> MHRRGVGAGAIAKKKLAEAKYKERGTVLAEDQLAQMSKQLDMFKTNLEEFASKHKQEIRKNPEFRVQFQDMCATIGVDPLASGKGFWSEMLGVGDFYYELGVQIIEVCLALKHRNGGLITLEELHQQVLKGRGKFAQDVSQDDLIRAIKKLKALGTGFGIIPVGGTYLIQSVPAELNMDHTVVLQLAEKNGYVTVSEIKASLKWETERARQVLEHLLKEGLAWLDLQAPGEAHYWLPALFTDLYSQEI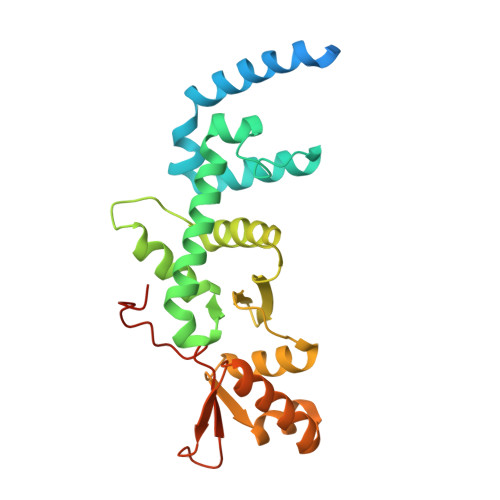TAEEAREALP> SNAERDEVGARKNAVDEEIERLSQPGGSEDQRLNALAERFGGVLLSEIYDDVSLEDAP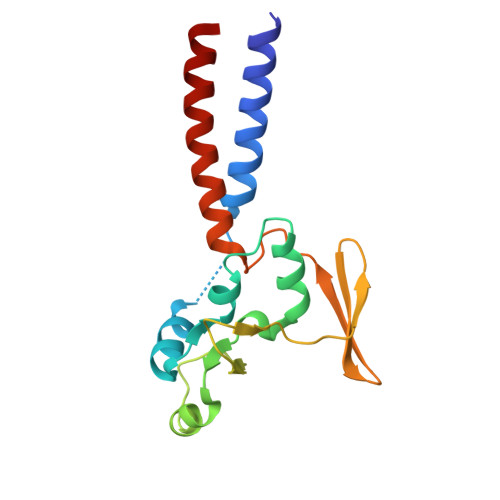YFSALYGPSRHAIVVPDLSQVTEHLEGLTDCPEDLYLIEGDPQSFDDSVFSVDELEKAVVVKIADRQWRYSRFPEVPLFGRAARESRIESLHAEREVLSERFATL>[2x]GMGSLAEWYQRIPTPDDLTRVESLFANMQAQFPQLKLEFK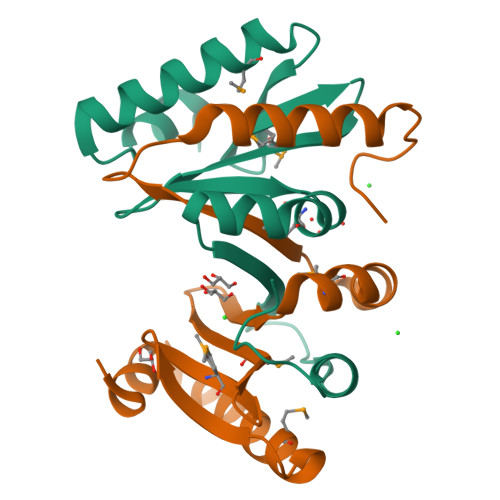WNQPMFTDHGTFIMGFNPSKKHLAVAIEPQTMTRFIPQIDKAGYDHSQIIRFPWHKPLDEQLIHDLIAYTIDQKKDATTFWQR>MVSKIIDIKTSIIKIPLKRTFITAVRSTNHIDSLAVELTLDNGVKGYGVAPATTAITGDTLQGMQYIIREIFAPVILGSDLSDYKQTLELAFKKVMFNSAAKMAIDLAYHDLLAKEQDISVAKLLGAKANSIVTDVSISCGNVAETIQNIQNGVEANFTAIKVKTGADFNRDIQLLKALDNEFSKNIKFRFDANQGWNLAQTKQFIEEINKYSLNVEIIEQPVKYYDIKAMAEITKFSNIPVVADESVFDAKDAERVIDEQACNMINIKLAKTGGILEAQKIKKLADSAGISCMVGCMMESPAGILATASFALAEDITVADLDPLDWVAKDLYSDYITFNEPNIILKDNLKGFGFNLAENLYFQSHHHHH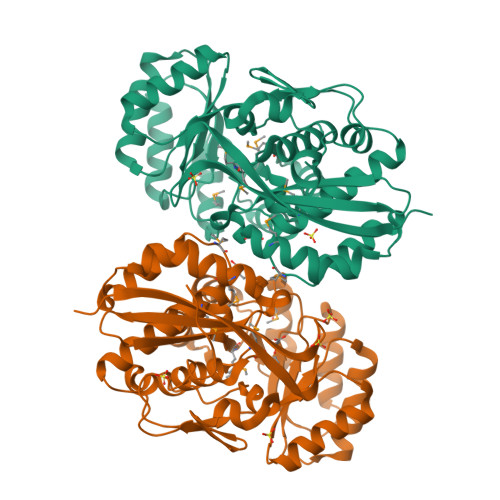HWSHPQFEK[2x]> MVTKDSIIRDLERENVGPEFGEFLNTLQTDLNSEKPPIEQVKSQLETHFNLAHETQEFSRKNDNAPVDKLLTNYYNNYEVNVLEFVLQMGFSRDLSIPLNVWFVLDMISQLSTSKQDLPLDYYLVLNNSQTGKYSDFVRYLIYEAVGAEIHCFEQGSMPEQYRSSRWEDKVKGPALANRGPIRGNVGAGDRKITFHLLCKKTARMILVGDDRETDFEMSDRSFVTLLLDYYQRVGTTKKIDLLLLTNNFDTNMNNKLQQLKILESLNMLKSNCYVLD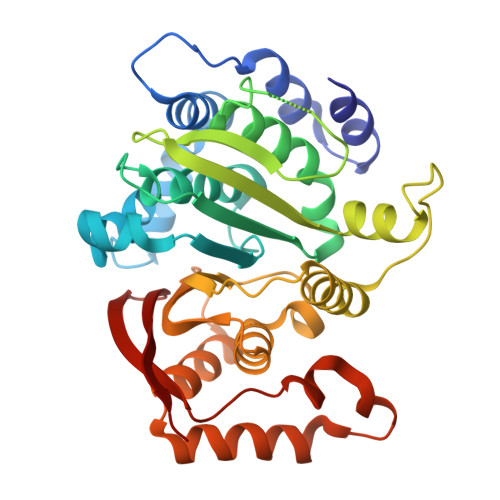YQITVDQVTANFNSYVEGIPAFRRHEIANFLKKRKTPKNADELIFKYVGRWNICYQKKFHQGNISIHQISGYLD>MAKKVKKYIVVESPAKAKTIKSILGNEYEVFASMGHIIDLPKSKFGVDLEKDFEPEFAVIKGKEKVVEKLKDLAKKGELLIASDMDREGEAIAWHIARVTNTLGRKNRIVFSEITPRVIREAVKNPREIDMKKVRAQLARRILDRIVGYSLSPVLWRNFKSNLSAGRVQSATLKLVCDREREILRFVPKKYHRITVNFDGLTAEIDVKEKKFFDAETLKEIQSIDELVVEEKKVSVKKFAPPEPFKTSTLQQEAYSKLGFSVSKTMMIAQQLYEGVETKDGHIAFITYMRTDSTRVSDYAKEEARNLITEVFGEEYVGSKRERRKSNAKIQDAHEAIRPTNVFMTPEEAG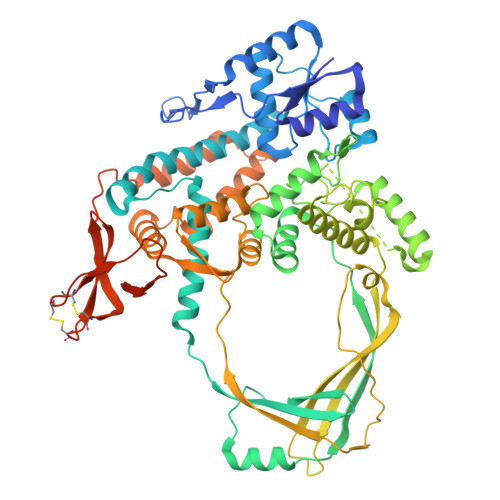KYLNSDQKKLYELIWKRFLASQMKPSQYEETRFVLRTKDGKYRFKGTVLKKIFDGYEKVWKTERNTGEFPFEEGESVKPVVVKIEEQETKPKPRYTEGSLVKEMERLGIGRPSTYASTIKLLLNRGYIKKIRGYLYPTIVGSVVMDYLEKKYSDVVSVSFTAEMEKDLDEVEQGKKTDKIVLREFYESFSSVFDRNDRIVVDFPTNQKCSCGKEMRLSFGKYGFYLKCECGKTRSVKNDEIAVIDDGKIFLGRKDSESGSPDGRSVEGKGNLSEKRRKGKKGS[2x]>SLRSDLINALYDENQKYDVCGIISAEGKIYPLGSDTAVLSTIFELFSRPIINKIAEKHGYIVEEPKQQNHYPDFTLYKPSEPNKKIAIDIKTTYTNKENEKIKFTLGGYTSFIRNNTKNIVYPFDQYIAHWIIGYVYTRVATRKSSLKTYNINELNEIPKPYKGVKVFLQDKWVIAGD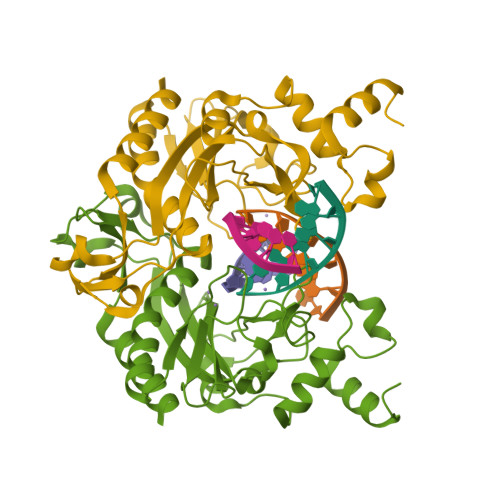LAGSGNTTNIGSIHAHYKDFVEGKGIFDSEDEFLDYWRNYERTSQLRNDKYNNISEYRNWIYRGRK[2x]> GPGSDDEINAQSVWSEEISSNYPLC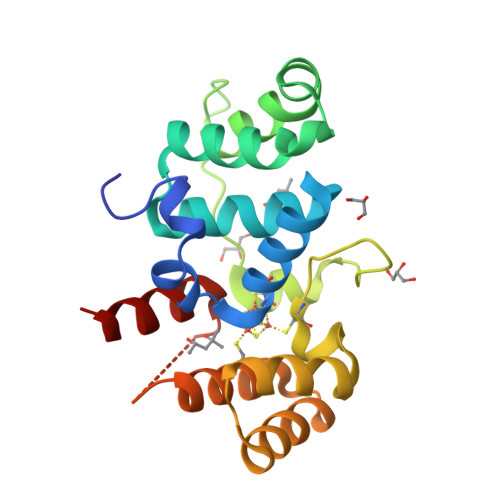IKNLMEGLKKNHHLRFFGRQQLSLFLKGIGLSADEALKFWSEAFTRNGNMTMEKFNKEFRFSFRHNYGLEGNRINFKPWDCHTILSKPRPGRGDYHGCPFRDWSHERLSAELRSMKLTQAQIISVLDSCQKGEYTIACTKVFEMTHNSASADLEIGEQTHIAHPNLYFERSRQLQK>HHHHHHFNLPPGNYKKPKLLYCSNGGHFLRILPDGTVDGTRDRSDQHIQLQLSAESVGEVYIKSTETGQYLAMDTDGLLYGSQTPNEECLWLERLEENHYNTYISKKHAEKNWFVGLKKNGSCKRGPRTHYGQKAIL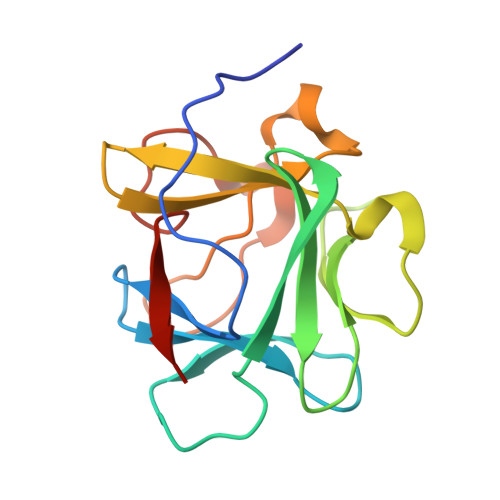FLPLPVSSD[2x]> MGNCNKPPKRPPNTQTSSNQPSAEFRRTAPPSLYGRYNCKCCWFADTNLITCNDHYLCLRCHQTMLRNSELCHICWKPLPTSITVPVEPSA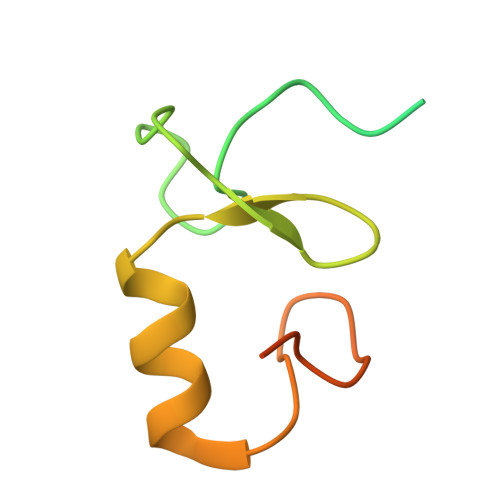PPP> HPETLVKVKDAEDQLGGRVGYIELDLASGKILESFRPEERFPMMSTFKVLLCGAVLSRVDAGQEQLGRRIHYSQNDLVKYSPVTEKHLTDGMTVGELCSAAITMSDNTAANLLLTTIGGPKELTAFLHNMGDHVTRLDRWEPELNEAIPNDERDTTTPVAMATTLRKLLTGELLTAASRQQLIDWMEADKVAGPLLRSALPAGWFIADKS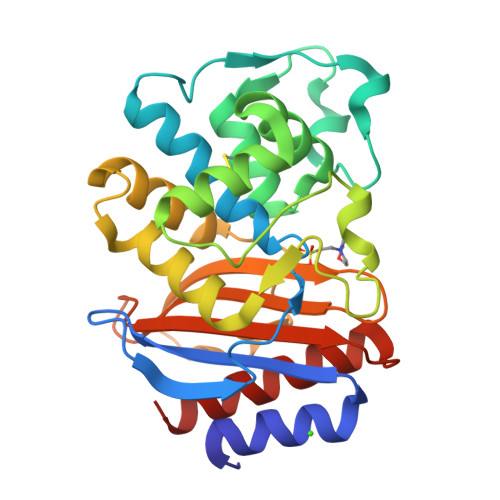GASERGSRGIIAALGPDGKPSRIVVIYMTGSQATMDERNRQIAEIGASLIKHW>MAVNVNTNVSAMTAQRYLTSATNAQQSSMERLSSGYKINSAKDDAAGLQISNRLNVQSRGLGVAVRNANDGISMAQTAEGAMKETTNILQRMRDLSLQSANGSNSKADRVAIQEEITALNDELNRVAETTSFGGNKLLNGTFATKSFQIGADNGEAVMLNIKDMRSDNALMGGKTYQAANGKDKNWGVEAGKTDLTITLKDKREGDVTISINAKEGDDIEELATYINGQTDMIKASVDEEGKLQLFTDNNRIDGAATFGGALAGELGIGAAQDVTVDTLDVTTVGGAQ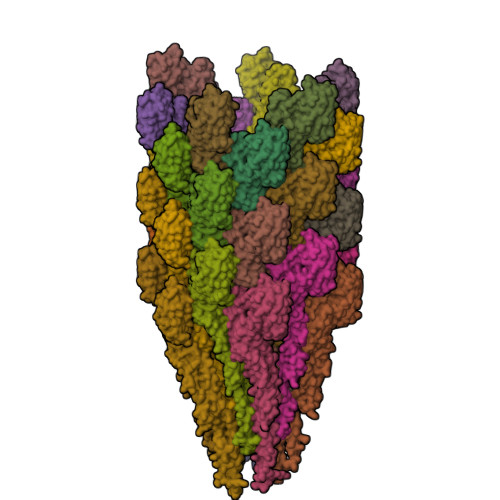ESVAIVDAALKYVDSHRAELGAFQNRFNHAINNLDNINENVNASKSRIKDTDFAKETTALTKAQILSQASSSVLAQAKQAPNSALALLG[33x]>NLRASAQARFATDAKAAAVQVLERRSAEVLKSEIVPALSPYKDAPLDPDNPSGNWRSFYFVDYYFSCPTRVAPSPKQRGGSVANLRPGLTCSGTETIFGIPVAWDIRGENGILGEGVVTVVVTATHPRGPKVTLGRRVTCYDVYPSP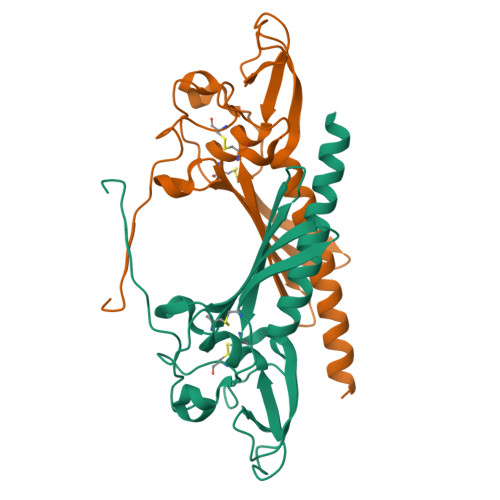TQDQPAPCPPPGGGRPGSGSWSHPQFEK[4x]>SPILGYWKIKGLVQPTRLLLEYLEEKYEEHLYERDEGDKWRNKKFELGLEFPNLPYYIDGDVKLTQSMAIIRYIADKHNMLGGCPKERAEISMLEGAVLDIRYGVSRIAYSKDFETLKVDFLSKLPEMLKMFEDRLCHKTYLNGDHVTHPDFMLYDALDVVLYMDPMCLDAFPKLVCFKKRIEAIPQIDKYLKSSKYIAWPLQGWQATFGGGDHPPKSDEFVIEKSLNRIKKFWKEAQYEVIEHSSGLKLVREWDVLEQACKEDLEELVSMKASNYYKIFEQDCLDLESKLTKLSEIQVNWVEVQFYWLDLYGILGENLDIQNFLPLETSKFKSLTSEYKMITTRAFQLDTTIEVIHIPNFDTTLKLTIDSLKMIKSSLSTFLERQRRQFPRFYFLGNDDLLKIIGSGKHHDQVSKFMKKMFGSIESIIFLEDFITGVRSVEGEVLNLNEKIELKDSIQAQEWLNILDTEIKLSVFTQFRDCLGQIKDGTDIEVVVSKYIFQAILLSAQVMWTELVEKCLQTNQFSKYWKEVDMKIKGLLDKLNKSSDNVKKKIEALLVEYLHFNNVIGQLKNCSTKEEARLLWAKVQKFYQKNDTLDDLNSVFISQSGYLLQYKFEYIGIPERLIYTPLLLIGFATLTDSLHQKYGGCFFGPAGTGKTETVKAFGQNLGRVVVVFNCDDSFDYQVLSRLLVGITQIGAWGCFDEFNRLDEKVLSAVSANIQQIQNGLQVGKSHITLLEEETPLSPHTAVFITLNPGYNGRSELPENLKKSFREFSMKSPQSGTIAEMILQIMGFEDSKSLASKIVHFLELLSSKCSSMNHYHFGLRTLKGVLRNCSPLISEFGEGEKTVVESLKRVILPSLGDTDELVFKDELSKIFDSAGTPLNSKAIVQCLKDAGQRSGFSMSEEFLKKCMQFYYMQKTQQALILVGKAGCGKTATWKTVIDAMAIFDGHANVVYVIDTKVLTKESLYGSMLKATLEWRDGLFTSILRRVNDDITGTFKNSRIWVVFDSDLDPEYVEAMNSVLDDNKILTLPNGERLPIPPNFRILFETDNLDHTTPATITRCGLLWFSTDVCSISSKIDHLLNKSYEALDNKLSMFELDKLKDLISDSFDMASLTNIFTCSNDLVHILGVRTFNKLETAVQLAVHLISSYRQWFQNLDDKSLKDVITLLIKRSLLYALAGDSTGESQRAFIQTINTYFGHDSQELSDYSTIVIANDKLSFSSFCSEIPSVSLEAHEVMRPDIVIPTIDTIKHEKIFYDLLNSKRGIILCGPPGSGKTMIMNNALRNSSLYDVVGINFSKDTTTEHILSALHRHTNYVTTSKGLTLLPKSDIKNLVLFCDEINLPKLDKYGSQNVVLFLRQLMEKQGFWKTPENKWVTIERIHIVGACNPPTDPGRIPMSERFTRHAAILYLGYPSGKSLSQIYEIYYKAIFKLVPEFRSYTEPFARASVHLYNECKARYSTGLQSHYLFSPRELTRLVRGVYTAINTGPRQTLRSLIRLWAYEAWRIFADRLVGVKEKNSFEQLLYETVDKYLPNQDLGNISSTSLLFSGLLSLDFKEVNKTDLVNFIEERFKTFCDEELEVPMVIHESMVDHILRIDRALKQVQGHMMLIGASRTGKTILTRFVAWLNGLKIVQPKIHRHSNLSDFDMILKKAISDCSLKESRTCLIIDESNILETAFLERMNTLLANADIPDLFQGEEYDKLLNNLRNKTRSLGLLLDTEQELYDWFVGEIAKNLHVVFTICDPTNNKSSAMISSPALFNRCIINWMGDWDTKTMSQVANNMVDVIPMEFTDFIVPEVNKELVFTEPIQTIRDAVVNILIHFDRNFYQKMKVGVNPRSPGYFIDGLRALVKLVTAKYQDLQENQRFVNVGLEKLNESVLKVNELNKTLSISLVKSLTFEKERWLNTTKQFSKTSQELIGNCIISSIYETYFGHLNERERADMLVILKRLLGKFAVKYDVNYRFIDYLVTLDEKMKWLECGLDKNDYFLENMSIVMNSQDAVPFLLDPSSHMITVISNYYGNKTVLLSFLEEGFVKRLENAIRFGSVVIIQDGEFFDPIISRLISREFNHAGNRVTVEIGDHEVDVSGDFKLFIHSCDPSGDIPIFLRSRVRLVHFVTNKESIETRIFDITLTEENAEMQRKREDLIKLNTEYKLKLKNLEKRLLEELNNSQGNMLENDELMVTLNNLKKEAMNIEKKLSESEEFFPQFDNLVEEYSIIGKHSVKIFSMLEKFGQFHWFYGISIGQFLSCFKRVFIKKSRETRAARTRVDEILWLLYQEVYCQFSTALDKKFKMIMAMTMFCLYKFDIESEQYKEAVLTMIGVLSESSDGVPKLTVDTNNDLRYLWDYVTTKSYISALNWFKNEFFVDEWNIADVVANSDNNYFTMASERDVDGTFKLIELAKASKESLKIIPLGSIENLNYAQEEISKSKIEGGWILLQNIQMSLSWVKTYLHKHVEETKAAEEHEKFKMFMTCHLTGDKLPAPLLQRTDRFVYEDIPGILDTVKDLWGSQFFTGKISGVWSVYCTFLLSWFHALITARTRLVPHGFSKKYYFNDCDFQFASVYLENVLATNSTNNIPWAQVRDHIATIVYGGK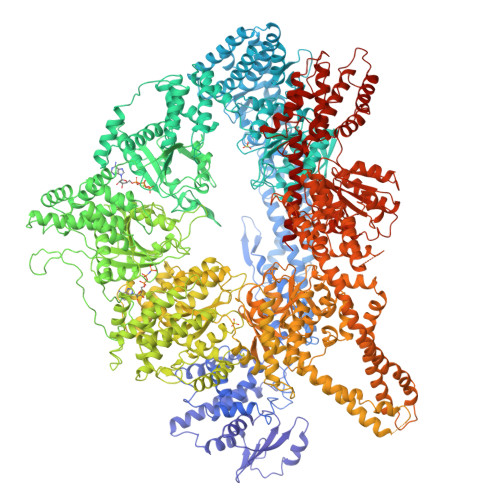IDEEKDLEVVAKLCAHVFCGSDNLQIVPGVRIPQPLLQQSEEEERARLTAILSNTIEPADSLSSWLQLPRESILNYERLQAKEVASSTEQLLQEM[2x]3-(2-bromophenoxy)pyridazine | C10 H7 Br N2 O 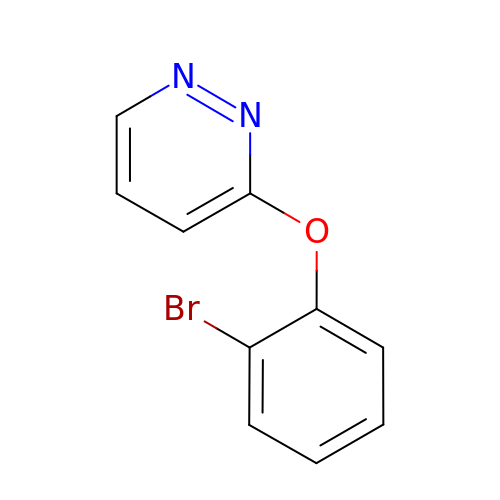| PESLFQDAIUALFG-UHFFFAOYSA-N> 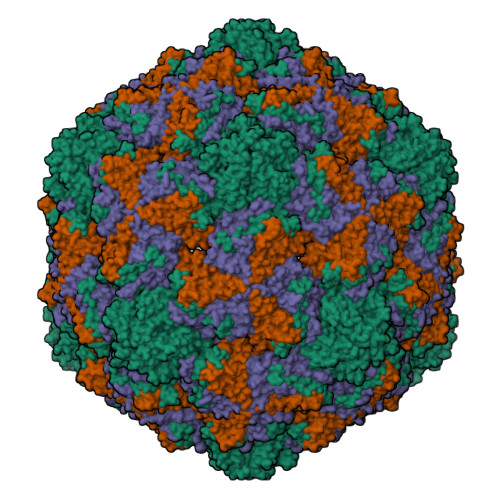NYHSRSESTVENFLCRSACVFYTTYRNHGTDGDNFGYWVINTRQVAQLRRKLEMFTYARFDLELTFVITSTQEQSTIQGQDSPVLTHQIMYVPPGGPVPTKVNSYSWQTSTNPSVFWTEGSAPPRMSIPFISIGNAYSMFYDGWAKFDKQGTYGINTLNNMGTLYMRHVNDGSPGPIVSTVRIYFKPKHVKTWVPRPPRLCQYQKAGNVNFEPTGVTESRTDITTMQ;> RVRSITLGNSTITTQECANVVVGYGVWPTYLNDDEATAEDQPTQPDVATCRFYTLESVMWQQSSPGWWWKFPDALSNMGLFGQNMQYHYLGRAGYTVHVQCNASKFHQGCLLVVCVPEAEMGCATLANKPDQKSLSNGETANMFESQNSTGQTAVQANVINAGMGVGVGNLTIFPHQWINLRTNNSATIVMPYINSVPMDNMFRHNNFTLMIIPFAPLSYSTGATTYVPITVTVAPMCAEYNGLRLA;> GLPTMLTPGSNQFLTSDDFQSPSAMPQFDVTPEMDIPGQVNNLMEIAEVDSVVPVNNTEGKVLSIESYQIPVQSNSTNGSQVFGFPLMPGASSVLNRTLLGEILNYYTHWSGSIKLTFMFCGSAMATGKFLLAYSPPGAGAPTTRKEAMLGTHVIWDVGLQSSCVLCIPWISQTHYRYVVVDEYTAGGYITCWYQTNIVVPADTQSDCKILCFVSACNDFSVRMLKDTPFIKQDNFYQ> SNAGSQPKLTEAVSLMEANIEEPLSTDDIAY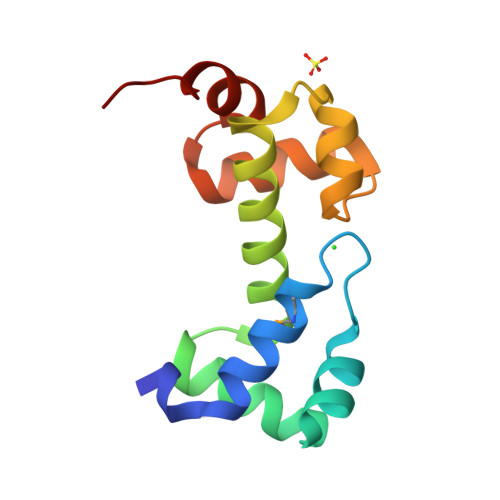YVGVSRRQLERLFKQYLGTVPSKYYLELRLNRARQLLQQTSKSIVQIGLACGFSSGPHFSSTYRNHFNITPREERAQRAQPG> MAFSELLDLVGGLGRFQVLQTMALMVSIMWLCTQSMLENFSAAVPSHRCWAPLLDNSTAQASILGSLSPEALLAISIPPGPNQRPHQCRRFRQPQWQLLDPNATATSWSEADTEPCVDGWVYDRSIFTSTIVAKWNLVCDSHALKPMAQSIYLAGILVGAAACGPASDRFGRRLVLTWSYLQMAVMGTAAAFAPAFPVYCLFRFLLAFAVAGVMMNTGTLLMEWTAARARPLVMTLNSLGFSFGHGLTAAVAYGVRDWTLLQLVVSVPFFLCFLYSWWLAESAR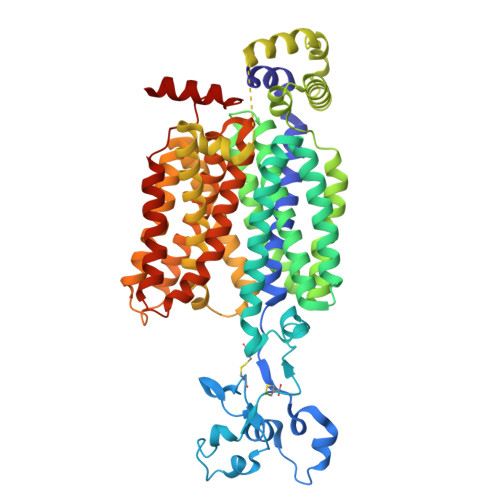WLLTTGRLDWGLQELWRVAAINGKGAVQDTLTPEVLLSAMREELSMGQPPASLGTLLRMPGLRFRTCISTLCWFAFGFTFFGLALDLQALGSNIFLLQMFIGVVDIPAKMGALLLLSHLGRRPTLAASLLLAGLCILANTLVPHEMGALRSALAVLGLGGVGAAFTCITIYSSELFPTVLRMTAVGLGQMAASGGAILGPLVRLLGVHGPWLPLLVYGTVPVLSGLAALLLPETQSLPLPDTIQDVQNQAVKKA> PLREGRGLGPLQIWQTDFTLEPRMAPRSWLAVTVDTASSAIVVTQHGRVTSVAAQHHWATAIAVLGRPKAIKTDNGSCFTSKSTREWLARWGIAHTTGIPGNSQGQAMVERANRLLKDKIRVL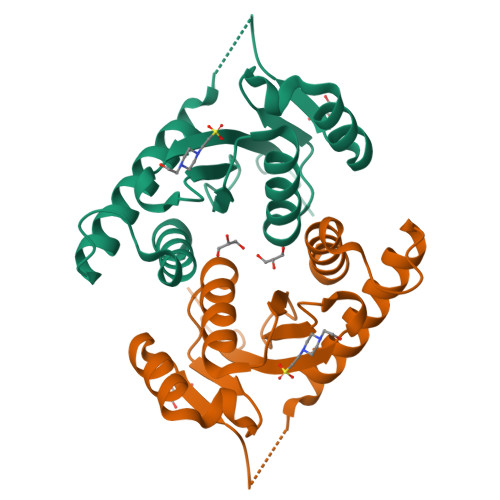AEGDGFMKRIPTSKQGELLAKAMYALNHFERGENTKTNL> XXXXXXXXXXXXXXXXXXXXXXXXXXXXXXXXXXXXXXXXXXXXXLERYRADLIDRKILRNKDHGVRAFAACCLSDILRLYAPDAPYTDKELTEIFRLFLAQLKLLQEPENGYLTQQTYLINNLLEYRSIVILTDLPSSSQLVEELFNIFYSPTNSTIQGNMFTAIGGILGEVISECDSLPMSALKMVFNKFLSHKRAESLDGINYKKDPGFEISLIICQTYSNRLGRHFIKFYSEIMYEVLGESDIHEKGIASSAYKTLVKIGNLTSELWKYAPELVGSVTGLLYQLLCSDNELFRESATKCVSKMLGTHSLINFAVAHSDTYKIWLSKMADISPHVRQAWVSEIPSILMSRSDLSDDISKGLAKALIDSDHTVRLSAIQTFHEVPVKRLWECLPNAAVFAGLVHLTRETRRDLRDECIDAVARIYTESIESIPKTNENKEIWGVVETIPSACFNLYYINDLEINMKVDLLTFEKFLPLGLSNEEFVQRLLTLLQGFNEKAFSSFYAFNRRQDQMSTVLWKFIEFCEETNSQSPAASLSDTKLIKTVEWISSGFPSHLNVEQILLAFRELN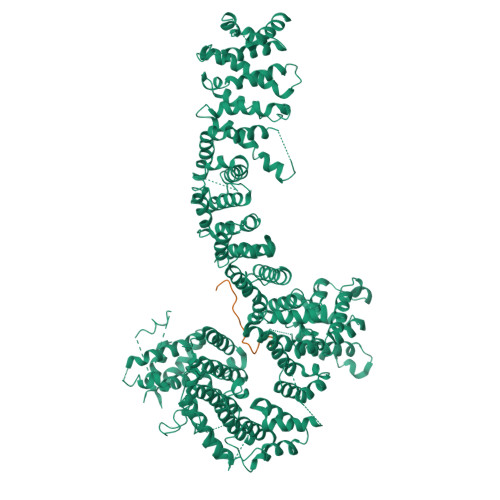DRRLYRLIKVAVAETSKHLTVRNAVSELFKRLEEPELFRKKNIKIESRFTRDNFSTVFRVLIYRAAPIIFNISNLPSFLNTSDSSNEDEKALKRQLIDNISIIKPGIFKDQVKNLVTIITEGETTGPGNTLSLAEAMRTVYKISKDKREHLDIEENTFFFQKLEDYAKEGNPLEAKYAIKLLGLAPNAAEYLSEVATAILPLDLKSKHFASNVLVLAEITKMQPQLLEKDSTEIVGLLIKDVLLSNDVVGDEDDQQAWFSDEDIYTGKADALSAKVFSLKLFANKIKVMAPDAHADEMTHAFTERTLKLFFYLVASGGELVSESNTDNYPTPANYQNKLRCCAGLHILKITKIASLSRFIKPQDISKLMNLVEDESLEVRSSFIGRLKDFLGDGSISIKFLPLVFFTAYEPDQALRTSTKMWINYTLSKENFRKGTFFERALPRLIHFIAHHPDVAEGLRLRETAFLTGLTTAIDYLVFYADSVLKASNLALLYYLAGRVRQYXXXXXXXXXXXXXXXXXXXXXXXXXXXXXXXXXXXXXXXXXXXXXXXXXXXXXXXXXX;> LTNPSQYLLQDAVTEREVLLVP> PAQDNSRFVIRDRNWHPKALTPDYKTSIARSPRQALVSIPQSISETTGPNFSHLGFGAHDHDLLLNFNNGGLPIGERIIVAGRVVDQYGKPVPNTLVEMWQANAGGRYRHKNDRYLAPLDPNFGGVGRCLTDSDGYYSFRTIKPGPHPWRNGPNDWRPAHIHFGISGPSIATKLITQLYFEGDPLIPMCPIVKSIANPEAVQQLIAKLDMNNANPMDCLAY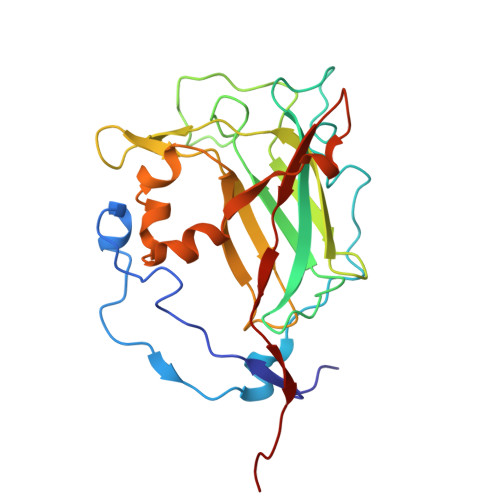RFDIVLRGQRKTHFENC> MTPASYNLAVRRAAPAVVNVYNRGLNTNSHNQLEIRTLGSG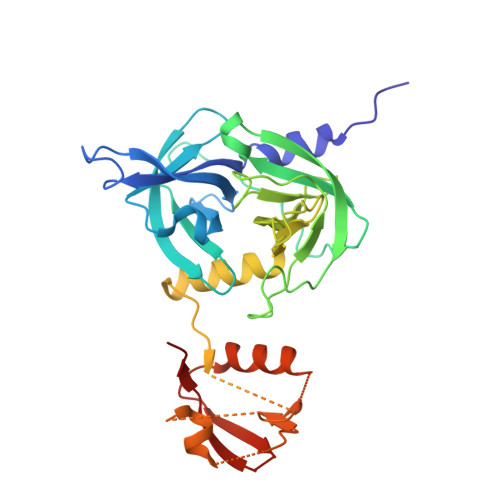VIMDQRGYIITNKHVINDADQIIVALQDGRVFEALLVGSDSLTDLAVLKINATGGLPTIPINARRVPHIGDVVLAIGNPYNLGQTITQGIISATGRIGLNPTGRQNFLQTDASINHGNSGGALVNSLGELMGINTLSFDKSNDGETPEGIGFAIPFQLATKIMDKLIRDGRVIRGYIGIGGREIAPLHAQGGGIDQLQGIVVNEVSPDGPAANAGIQVNDLIISVDNKPAISALETMDQVAEIRPGSVIPVVVMRDDKQLTLQVTIQEYPATN>[2x]SNAMNHSRESYDRLARELGGYRHPWARVLSGPDPELTFDLWLSRLLTPQTRVLEAGCGHGPDAARFGPQAARWAAYDFSPELLKLARANAPHADVYEWNGKGELPAGLGAPFGLIVS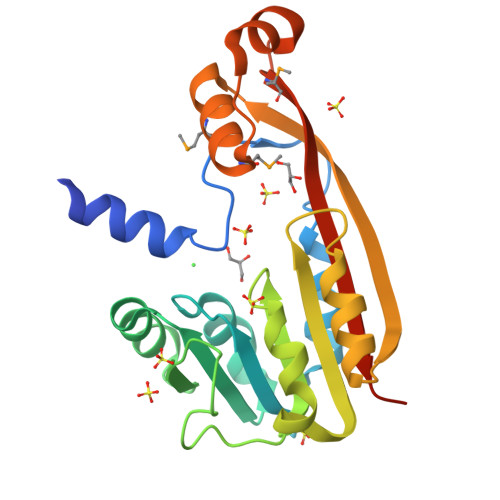RRGPTSVILRLPELAAPDAHFLYVGPRLNVPEVPERLAAVGWDIVAEDHVSVLAHAPTWEDWQMRGEFMGKLARRADWDAEATVRGMPYREERHLVLARQLGVARKLGA> MPRLVALVKGRVQGVG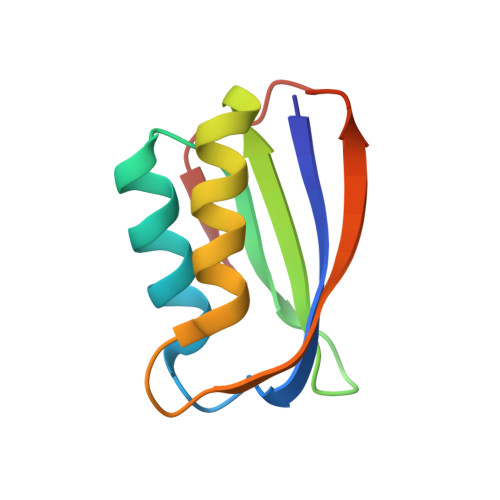YRAFAQKKALELGLSGYAENLPDGRVEVVAEGPKEALELFLHHLKQGPRLARVEAVEVQWGEEAGLKGFHVY McrBC is a two-component MDRS that in Escherichia coli (Ec) restricts phage DNA and foreign DNA containing methylated cytosines. EcMcrB consists of an N-terminal DNA-binding domain that targets fully or hemi-methylated RMC sites (where R is a purine base and MC is a 4-methyl-, 5-methyl-, or 5-hydroxymethyl-cytosine), and a C-terminal AAA+ (extended ATPases Associated with various cellular Activities) domain that hydrolyzes GTP and oligomerizes into hexamers. Biochemical data suggest that stimulated GTP hydrolysis powers DNA translocation, allowing EcMcrBC complexes bound to distant RMC sites to interact and induce cleavage on both strands. Here, we present cryo-EM structures of an McrB hexamer and McrBC complexes from the evolutionarily distant archaeal species Thermococcus gammatolerans (Tg) and the well-characterized E. coli system.

In parallel, we also determined the structure of TgMcrBAAA in the presence of GTPγS by X-ray crystallography at 2.95-Å resolution. Symmetry-related hexamers abut against each other in the crystal lattice, deforming the planar arrangement of the six subunits in each molecule. This produces an “open-ring” conformation in which the subunits at the loose A/B interface are significantly splayed apart, and the small subdomain of the F subunit becomes highly disordered. The individual TgMcrBAAA monomers, however, adopt the same overall conformation and organization of nucleotide binding, as is observed in the cryo-EM reconstruction. The distorted appearance of the crystallographic hexamer suggests a greater flexibility at the loose interfaces, which could more readily be influenced by crystal packing forces. The asymmetry in the ring also explains how crystal packing forces could induce and/or sustain the open conformation observed in our TgMcrBAAA X-ray structure, as the loose interfaces likely have a greater propensity for flexibility resulting from the fewer stabilizing interactions. Our cryo-EM and X-ray structures of TgMcrBAAA reveal that Arg425 is not only important for stabilizing Glu375 in cis as predicted from the previous structures of E. coli complexes, but also interacts with the phosphates of GTP in trans.

>[6x]MNESAGHNIKEDYFRVDMLLNKKGQVILYGPPGTGKTWIARKYVVEETNEKTPGNKWEFITFHQSYSYEEFIEGFRPRTDNEEKIRYVVEDGIFKKIALRALVKGLFELEDATIGKDKIHRLYILLTKKEPLSPTEYEEYLRLKRYLWELVGGLPKDKLKNLTPKFYLIIDEINRGNISKIFGELITLLEKDKRLGGENQLIVRLPYSGEPFAVPPNLYIIGTMNTADRSIALLDVALRRRFAFIEVEPRPEFLEKENLKKIREKKLKTEDRKRLNEKLNELFSKLGNDNYFLKTLLEKINVRITVVKDRDHRIGHSYFLNVETVEDLHHVWYYEVLPLLMEYFYNDWETIKWVLNEKGKEHGNVFFEKLRLTGPNGEEAYQLKVLEGDAFIGALKRIISKNTPSQEGGATTNEENSPENTQSQTEGD> MVDSIHRIASALDTAKVITREAAAVATSKLGESSYTYYSQNINPQQLVTLLNSRNSREVRDAMKRIISIMASDDDSIDVQLYFADVVKNITTNDTKVKRLIHLYLLRFAENDPNLTLLSINSLQKSLSDSNSELRCFALSALSDMKMSSLAPIILHTVKKLVTDPSAMVRGEVALAIIKLYRAGKNDYHEELLDILKELMADTDPKVISCAVLAYKECYADHLELLHGHFRRYCRIIKQLDSWSQSYLIELLIKYCKQYLPKPTVVDKSSEGSPRSCPLPDKYNEIEYPSYEVVNDPDLDLFLQSLNCLIYSSNPTVILSCCNALYQLASPLQMKNTKFIEALVRTVTMTENQGNKEMLLQAIHFLSILDQTLFLPYTKKFYVFPKDPIVASIWKIQILSTLINESNVKEIFKELKYYVASAHFPENVVIMAVKSLSRCGQLSTSWESHVMKWLIDHMESHNLSASVLDAYVNVIRMLVQKNPTKHLRIIFKLADLLTVQTSLADNARAGIVWLFGEIASIEFKICPDVLRRLIQNFSNEGPETRCQILVLSAKLLSYDIDNFKQAQVTGSEENNQNPPYYDFSGSRISQMYNAVLYLAKYDDEFDIRDRARMISSLFDSGKYEIVSLLLQAPKPTARSDDFIVSARLETHTPEIKEFFRMLPWNTEITEVG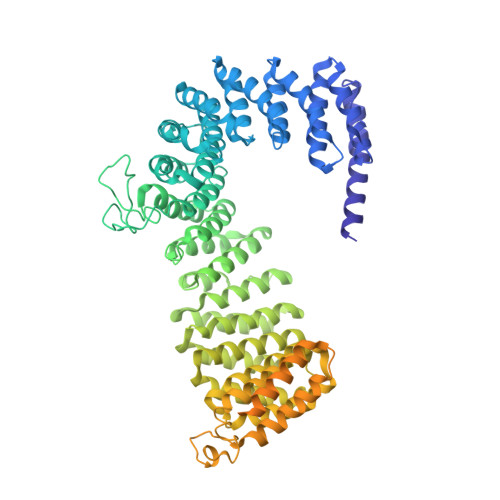ETGNDIREGAELKDYNKYKKSFSSQSFITNNSARSFTSSSNAKLTGINDGDSNSISGKGNVNTFTSQNGKKYRLQSLDEFFSDIPERKSKPRKIIKVVEESSDEDEDESEESSDDDEYSDSSLGTSSSGTSSSHLEL APP and its paralogues APP-like protein 1 (APLP1) and APP-like protein 2 (APLP2) contain the highly conserved heparan sulfate (HS) binding domain E2, which effects various (patho)physiological functions. The ectodomains of all APP-family proteins share the N-terminal E1 domain and the central E2 domain. Comparable to the E2 structures of other APP-family proteins, a coiled-coil-like fold is formed by helix αB (Gly302–Gln338) and the first half of helix αC (Lys344–Arg379). The C-terminal parts of helices αC (Val380–Leu399), αD (Ala406–Val437), αE (Pro439–Asp468) and αF (Pro471–Gly491) constitute a four-helix bundle.

To clarify these issues, we decided to co-crystallize APLP1 E2 in the presence of a heparin dodecasaccharide. The heparin–protein complex crystallized in space group P3121 with a very high solvent content of 77%. Refinement was performed to a resolution of 2.5 Å and resulted in good stereochemistry. In contrast to the apo form, the short N-terminal α-helix αA (Asp292–Phe298) is well defined in the electron-density map in this trigonal crystal form of the complex. The co-crystal structure contained an (APLP1 E2)2–(heparin)2 assembly and revealed two different heparin-binding modes of APLP1 E2. A second heparin chain is tightly and specifically bound with its nonreducing terminal Δ4UAp2S in the centre of the APLP1 E2 dimer. The longest heparin stretch of six sugar residues is exclusively associated with one APLP1 E2 protomer (chain b) and extends to a surface patch distant from the centre of the dimer. Only the register of the sugar moieties determines the fit to this surface patch, which thus seems to be compatible with the binding of continuous heparin chains in various sulfation states. Our structural data rather suggest specificity of APLP1 E2 for nonreducing ends of heparin and HS exposing terminal Δ4UAp2S and IdoAp2S, respectively.

>[2x]EAEFPTDGVDIYFGMPGEISEHEGFLRAKMDLEERRMRQINEVMREWAMADNQSKNLPKADRQALNEHFQSILQTLEEQVSGERQRLVETHATRVIALINDQRRAALEGFLAALQADPPQAERVLLALRRYLRAEQKEQRHTLRHYQHVAAVDPEKAQQMRFQVHTHLQVIEERVNQSLGLLDQNPHLAQELRPQIQELLHSEHLGPSEL>[4x]MVMAGASSLDEIRQAQRADGPAGIL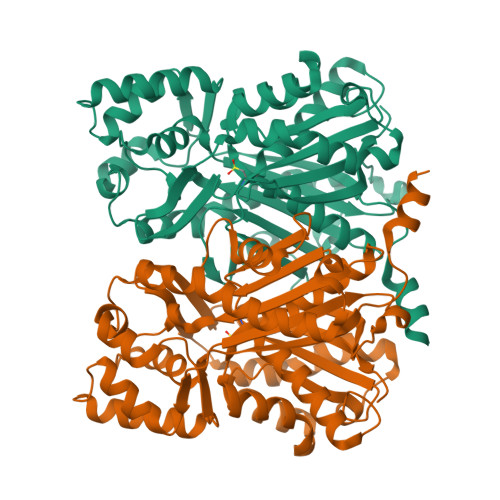AIGTANPENHVLQAEYPDYYFRITNSEHMTDLKEKFKRMCDKSTIRKRHMHLTEEFLKENPHMCAYMAPSLDTRQDIVVVEVPKLGKEAAVKAIKEWGQPKSKITHVVFCTTSGVDMPGADYQLTKLLGLRPSVKRLMMYQQGCFAGGTVLRIAKDLAENNRGARVLVVCSEITAVTFRGPSDTHLDSLVGQALFSDGAAALIVGSDPDTSVGEKPIFEMVSAAQTILPDSDGAIDGHLREVGLTFHLLKDVPGLISKNIVKSLDEAFKPLGISDWNSLFWIAHPGGPAILDQVEIKLGLKEEKMRATRHVLSEYGNMSSACVLFILDEMRRKSAKDGVATTGEGLEWGVLFGFGPGLTVETVVLHSVPL> MNTQSLMSSTHTIAASDPHIQVMGRTHINDDASLTFGYPGVSLSTIVAGSRLTAEMQSSNGNSWIDVIIDNHPPTSIKLDAQQQTVELFHFPNSGEHRVEIIHRSENWHGQVTLKQLTLTGTQFLPAPVLPQRKILVLGDSVTCGEAIDRVAGEDKNTRWWNARESYGMLTAKALDAQVQLVCWGGRGLIRSWNGKTDDANLPDFYQFTLGDTGQAPQWDHHRYQPDLIISAIGTNDFSPGIPDRATYINTYTRFVRTLLDNHPQATIVLTEGAILNGDKKAALVSYIGETRQQLHSNRVFYASSSHHPGDNSDAHPTKDQHAAMARELTPQLRQIMDWLEHHHHHH

CE2 enzymes are acetyl esterases (that are generally not appended to other catalytic modules), which are reported to be active on synthetic aryl-esters and acetylated xylan. Here we report the biochemical properties and crystal structure of several CE2 members, both single-module CE2 enzymes and CtCE2, a component of CtCel5C-CE2. All three 3D structures reveal a bi-domain enzyme in which an N-terminal β-sheet “jelly roll” domain (around 130 residues) is linked to a C-terminal domain of approximately 220 residues. The C-terminal domains possess an atypical α/β-hydrolase (SGNH-hydrolase) fold, consisting of repeating β-α-β motifs that form a curved central five-stranded parallel β-sheet, in the strand order β2, β1, β3, β4, and β5 with strand β2 interrupted by loop insertion.

CjCE2A is a canonical serine hydrolase, with a classical Ser-His-Asp triad, in which Ser-160 is the catalytic nucleophile, His-335 activates the serine, and Asp-333 makes a hydrogen bond with Nδ1 of His-335 thus completing the catalytic triad. The oxyanion hole, which stabilises the incipient tetrahedral transition-state, comprise the N of Ser-160 and Gly-205 and the Nδ2 of Asn-255. Indeed, in the pocket within the cleft of CjCE2A is a formate molecule, mimicking the reactive intermediate, which makes hydrogen bonds with the residues that form the oxyanion hole. Based on their catalytic efficiencies, CtCE2 and CjCE2B exhibit a significant preference for acetylated glucomannan over xylan, whereas CjCE2A and CjCE2C do not distinguish between the two polysaccharides. Pull-down assays revealed that none of the Cellvibrio enzymes bound to insoluble cellulose. Although the two structurally characterised Cellvibrio esterases do not bind cellohexaose or cellulose, they do contain aromatic residues in the cleft that houses the active site. Thus, Tyr-665 in CtCE2 is conserved in the C. japonicus esterases (Trp-231 in CjCE2A and Tyr-206 in CjCE2B), while Trp-335 in CjCE2B is equivalent to Trp-790 in the Clostridium enzyme. To address this issue Tyr-683 and Trp-127, which are located in or at the interface, of the CBM-like domains of CtCE2 and CjCE2A, respectively, were mutated and the activities of the two esterase variants were assessed. It would appear, therefore, that the CBM-like domain contributes to substrate recognition in CjCE2A, but its role in the catalytic activity of CtCE2 is less evident.>[3x]GGEIRPTIGQQMETGDQRFGDLVFRQLAPNVWQHTSYLDMPGFGAVASNGLIVRDGGRV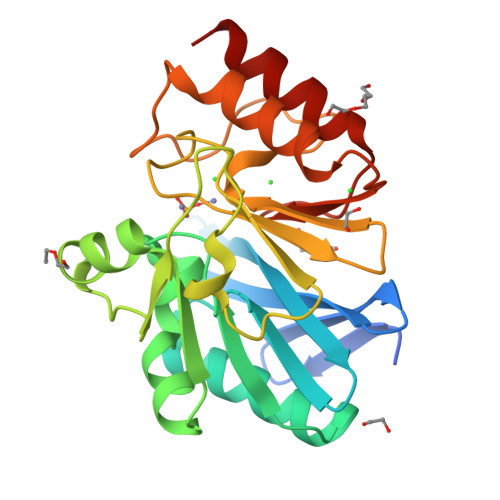LVVDTAWTDDQTAQILNWIKQEINLPVALAVVTHAHQDKMGGMDALHAAGIATYANALSNQLAPQKGMVAAQHSLTFAANGWVEPATAPNFGPLKVFYPGPGHTSDNITVGIDGTDIAFGGCLIKDSKAKSLGNLGDADTEHYAASARAFGAAFPKASMIVMSHSAPDSRAAITHTARMADKLR> V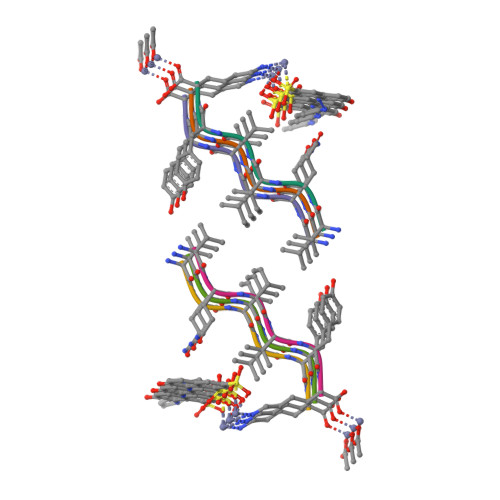QIVYK>[5x]EDPSLDRPFISEGTTLKDLIYDMTTSGSGSGLPLLVQRTIARTIVLQESIGK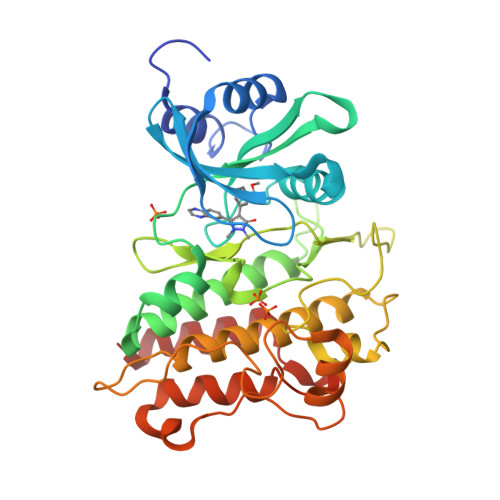GRFGEVWRGKWRGEEVAVKIFSSREERSWFREAEIYQTVMLRHENILGFIAADNKDNGTWTQLWLVSDYHEHGSLFDYLNRYTVTVEGMIKLALSTASGLAHLHMEIVGTQGKPAIAHRDLKSKNILVKKNGTCCIADLGLAVRHDSATDTIDIAPNHRVGTKRYMAPEVLDDSINMKHFESFKRADIYAMGLVFWEIARRCSIGGIHEDYQLPYYDLVPSDPSVEEMRKVVCEQKLRPNIPNRWQSCEALRVMAKIMRECWYANGAARLTALRIKKTLSQLSQQEGIKM> CDDFLDRQVPQGIVTGDQIASPEYVDNLVISAYAIWATGDDINSSFSLWNYDVRSDDCYKGGSGTEDGGVFNALEISKGINTTDWNINDIWKRLYQCITRANTALQSLDQMDEKTYPLKNQRIAEMRFLRGHAHFMLKQLFKKIVIVNDENMEPDAYNELSNTTYTN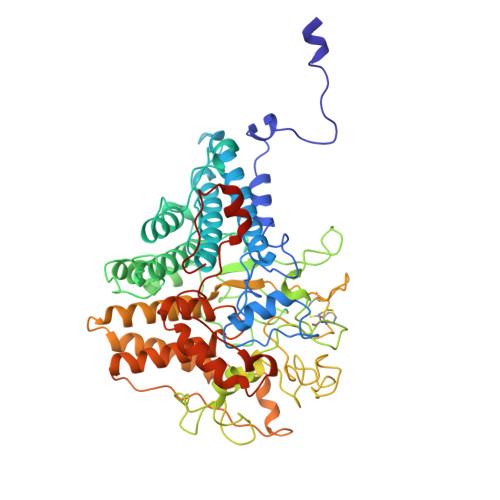DEQWQKIADDFQFAYDNLPEVQIEKGRPAQAAAAAYLAKTYLYKAYRQDGADNALTGINEEDLKQVVKYTDPLIMAKGGYGLETDYSMNFLPQYENGAESVWAIQYSINDGTYNGNLNWGMGLTTPQILGCCDFHKPSQNLVNAFKTDSQGKPLFSTYDNENYEVATDNVDPRLFHTVGMPGFPYKYNEGYIIQKNDDWSRSKGLYGYYVSLKENVDPDCDCLKKGSYWASSLNHIVIRYADVLLMRAEALIQLNDGRITDAISLINEVRSRAAGSTMLIFNYKEDYGVNFKVTPYDLKAYAQDEAMKMLKWERRVEFGMESSRFFDLVRWGEAKDVINAYYVTEASRCSIYKNAGFTENKNEYLPVPFEQISASNGNYTQNFGWAAAAHHHHHH>MVEQIKDKLGRPIRDLRLSVTDRCNFRCDYCMPKEVFGDDFVFLPKNELLTFDEMARIAKVYAELGVKKIRITGGEPLMRRDLDVLIAKLNQIDGIEDIGLTTNGLLLKKHGQKLYDAGLRRINVSLDAIDDTLFQSINNRNIKATTILEQIDYATSIGLNVKVNVVIQKGINDDQIIPMLEYFKDKHIEIRFIEFMDVGNDNGWDFSKVVTKDEMLTMIEQHFEIDPVEPKYFGEVAKYYRHKDNGVQFGLITSVSQSFCSTCTRARLSSDGKFYGCLFATVDGFNVKAFIRSGVTDEELKEQFKALWQIRDDRYSDERTAQTVANRQRKK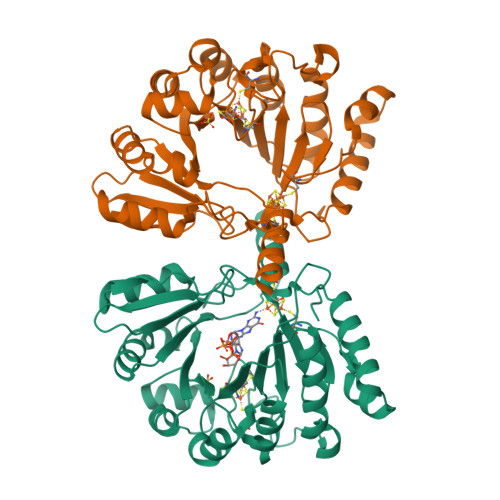INMNYIGG[2x]> IVGGTASVRGEWPWQVTLHTTSPTQRHLCGGSIIGNQWILTAAHCFYGVESPKILRVYSGILNQSEIKEDTSFFGVQEIIIHDQYKMAESGYDIALLKLETTVNYTDSQRPISLPSKGDRNVIYTDCWVTGWGYRKLRDKIQNTLQKAKIPLVTNEECQKRYR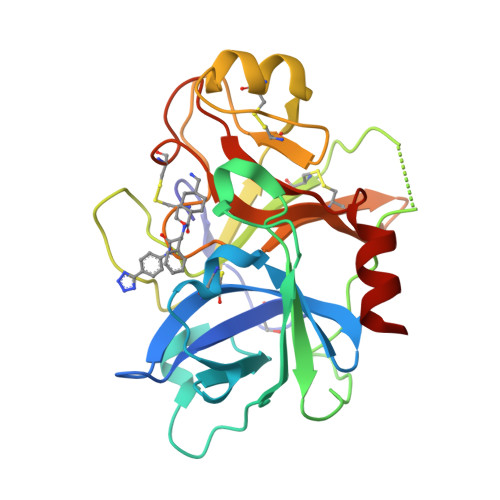GHKITHKMICAGYREGGKDACKGDSGGPLSCKHNEVWHLVGITSWGEGCAQRERPGVYTNVVEYVDWILEKTQAV> VDPDAKVDKVDYEIDYSTAGYSFWNEVNEEVKETTTIGKNDTEG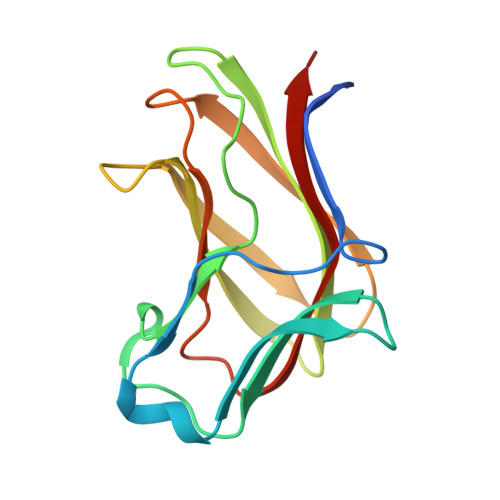CLEIKTSVAASQNHFIQYHTADNLPIEIGKEYKLKMMVRGSAEGKLNFGVGPWSGRAEGSFSFNTEWKEYEFSFKAVADGGHVMTQSGLFVGTIQIKYVKITHSEA> SATRELDELMASLSD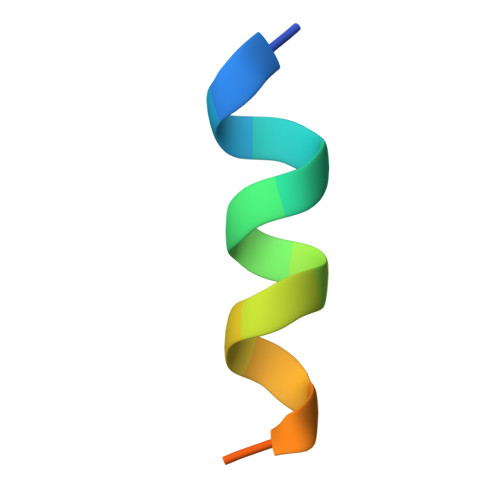FK>MCLEDSDAGASNEYDSSPAAWNKEDFPWSGKVKDILQNVFKLEKFRPLQLETINVTMAGKEVFLVMPTGGGKSLCYQLPALCSDGFTLVICPLISLMEDQLMVLKQLGISATMLNASSSKEHVKWVHAEMVNKNSELKLIYVTPEKIAKSKMFMSRLEKAYEARRFTRIAVDEVHCCSQWG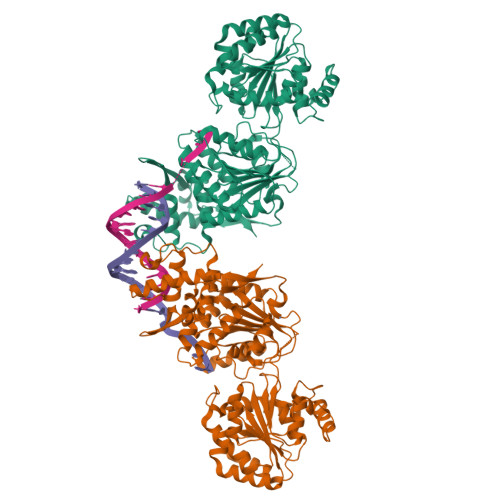HDFRPDYKALGILKRQFPNASLIGLTATATNHVLTDAQKILCIEKCFTFTASFNRPNLYYEVRQKPSNTEDFIEDIVKLINGRYKGQSGIIYCFSQKDSEQVTVSLQNLGIHAGAYHANLEPEDKTTVHRKWSANEIQVVVATVAFGMGIDKPDVRFVIHHSMSKSMENYYQESGRAGRDDMKADCILYYGFGDIFRISSMVVMENVGQQKLYEMVSYCQNISKCRRVLMAQHFDEVWNSEACNKMCDNCCKDSAFERKNITEYCRDLIKILKQAEELNEKLTPLKLIDSWMGKGAAKLRVAGVVAPTLPREDLEKIIAHFLIQQYLKEDYSFTAYATISYLKIGPKANLLNNEAHAITMQVTKSTQNSFRAESSQTCHSEQSDKKMEAENLYFQSHHHHHHDYKDDDDK[4x]Gelsolin is a 80 kDa protein displaying six homologous, gelsolin-like, domains (named G1 to G6) existing as two alternative splicing variants: a 24-residue shorter intracellular form and a variant secreted in the bloodstream. Both isoforms bind actin fibrils, severing the filaments and preventing repolymerization. Gelsolin, in particular, hosts eight calcium binding sites: one for each domain and two incomplete sites, which require actin contribution. Moreover, mutations in the gelsolin gene are directly responsible for gelsolin amyloidosis (GA) with 100% penetrance.

Here we report a structural and functional characterization of the isolated G2 domain of the N184K variant. Best diffracting crystals were used to determine N184K structure at 1.05 and 1.7 Å resolution, which will be hereafter referred as the orthorhombic and trigonal forms, respectively. Only few amino acids were not modeled: residues 260–266 at the N-terminus of the orthorhombic crystal form, and residues 256–266, 158–159 and the side chain of 169 in the trigonal crystal. In agreement with denaturation studies, electron density for Ca2+ was clearly visible in its binding site and the ion was refined to 100% occupancy in both structures. In the wt structure, the C-terminal tail is wrapped around the globular domain and is involved in extensive interactions with loops β2-β3 and β1-β2. More importantly, it provides a sort of lid for the calcium binding site, contributing to the hexacoordination of the ion with the side-chain of D259. In contrast, in the trigonal crystal the C-terminus dissociates from the Ca2+ coordination, assuming a stretched configuration. Such conformational change leaves the calcium ion solvent exposed, with a water molecule taking the place of the carboxylate of D259. Nevertheless, the calcium ion seems to be still firmly bound to the protein, as its B factor is comparable to those of the surrounding atoms. The open conformation of the C-terminus, observed in the trigonal crystal, is likely due to crystal packing: the terminal tail interacts with residues of the N-terminus and of the β3-β4 loop belonging to a symmetric molecule.

> GSHHVVPNEVVVQRLFQVKGRRVVRATEVPVSWESFKNGDCFILDLGNNIHQWCGSNSNRYERLKATQVSKGIRDNERSGRARVHVSEEGTEPEAMLQVLGPKPALPAGTEDTAKEDAA> MNNIWWQTKGQGNVHLVLLHGWGLNAEVWRCIDEELSSHFTLHLVDLPGFGRSRGFGALSLADMAEAVLQQAPDKAIWLGWALGGLVASQIALTHPERVQALVTVASSPCFSARDEWPGIKPDVLAGFQQQLSDDFQRTVERFLALQTMGTETA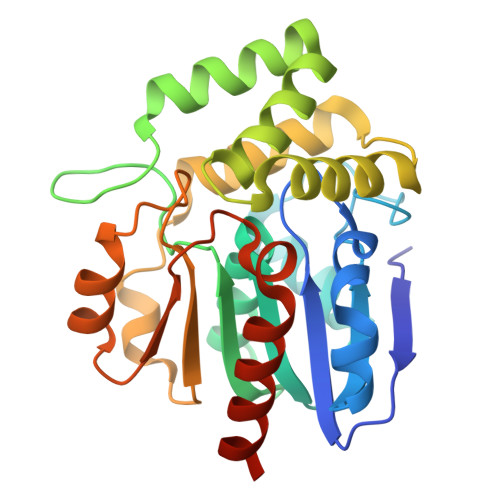RQDARALKKTVLALPMPEVDVLNGGLEILKTVDLRQPLQNVSMPFLRLYGYLDGLVPRKVVPMLDKLWPHSESYIFAKAAHAPFISHPAEFCHLLVALKQRVLEHHHHHH N-[(1R)-1-(2-chlorophenyl)propyl]-3-{4-[(1-methylpiperidin-4-yl)oxy]phenyl}-1H-indazole-5-carboxamide | 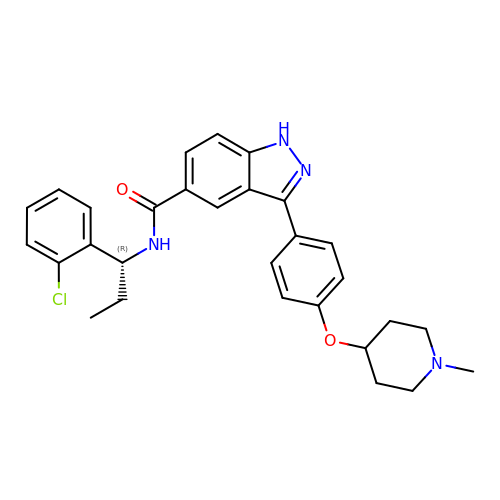C29 H31 Cl N4 O2 | XEADJJXUBNVGAN-AREMUKBSSA-N7-methyl-3-[[4-oxidanyl-1-[(3~{R},4~{R})-3-phenyl-1-[(5-pyrimidin-5-ylthiophen-2-yl)methyl]piperidin-4-yl]carbonyl-piperidin-4-yl]methyl]pyrrolo[2,3-d]pyrimidin-4-one 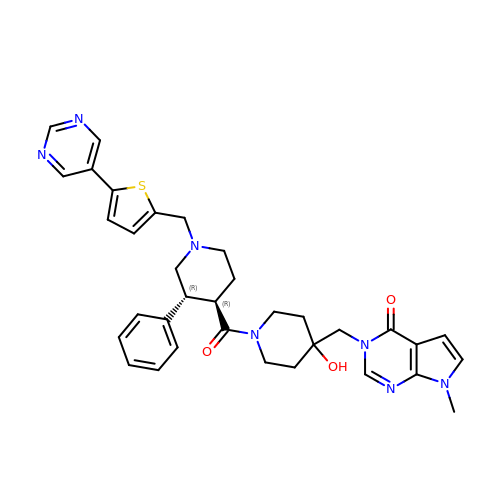| C34 H37 N7 O3 S | NZZFXHIASCZNOO-PXJZQJOASA-N~{N}-[4-(4-fluoranyl-2,6-dimethyl-phenoxy)-3-[2-[4-(2-hydroxyethyloxy)-3,5-dimethyl-phenyl]-5-methyl-4-oxidanylidene-furo[3,2-c]pyridin-7-yl]phenyl]ethanesulfonamide 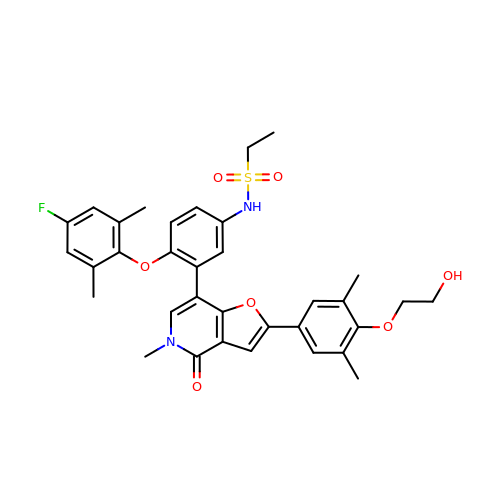| C34 H35 F N2 O7 S | FMOLFXOGJCZPJG-UHFFFAOYSA-N> MESHVKYLDELILAIKDLNSGVDSKVQIKKVPTDPSSSQEYAKSLKILNTLIRNLKDQRRNNIMKNDTIFSKTVSALALLLEYNPFLLVMKDSNGNFEIQRLIDDFLNISVLNYDNYHRIWFMRRKLGSWCKACVEFYGKPAKFQLTAHFENTMNLYEQALTEVLLGKTELLKFYDTLKGLYILLYWFTSEYSTFGNSIAFLDSSLGFTKFDFNFQRLIRIVLYVFDSCELAALEYAEIQLKYISLVVDY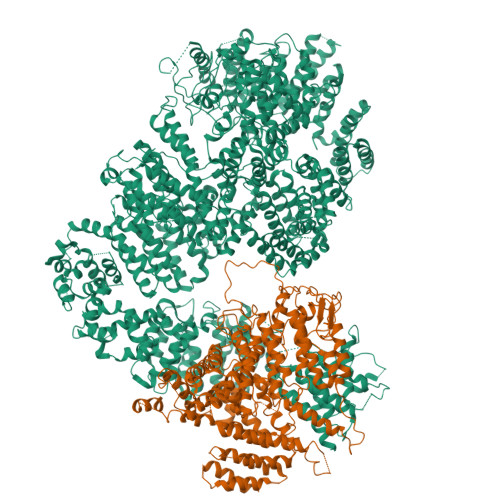VCNRTISTALDAPALVCCEQLKFVLTTMHHFLDNKYGLLDNDPTMAKGILRLYSLCISNDFSKCFVDHFPIDQWADFSQSEHFPFTQLTNKALSIVYFDLKRRSLPVEALKYDNKFNIWVYQSEPDSSLKNVTSPFDDRYKQLEKLRLLVLKKFNKTERGTLLKYRVNQLSPGFFQRAGNDFKLILNEASVSIQTCFKTNNITRLTSWTVILGRLACLESEKFSGTLPNSTKDMDNWYVCHLCDIEKTGNPFVRINPNRPEAAGKSEIFRILHSNFLSHPNIDEFSESLLSGILFSLHRIFSHFQPPKLTDGNGQINKSFKLVQKCFMNSNRYLRLLSTRIIPLFNISDSHNSEDEHTATLIKFLQSQKLPVVKENLVIAWTQLTLTTSNDVFDTLLLKLIDIFNSDDYSLRIMMTLQIKNMAKILKKTPYQLLSPILPVLLRQLGKNLVERKVGFQNLIELLGYSSKTILDIFQRYIIPYAIIQYKSDVLSEIAKIMCDGDTSLINQMKVNLLKKNSRQIFAVALVKHGLFSLDILETLFLNRAPTFDKGYITAYLPDYKTLAEITKLYKNSVTKDASDSENANMILCSLRFLITNFEKDKRHGSKYKNINNWTDDQEQAFQKKLQDNILGIFQVFSSDIHDVEGRTTYYEKLRVINGISFLIIYAPKKSIISALAQISICLQTGLGLKEVRYEAFRCWHLLVRHLNDEELSTVIDSLIAFILQKWSEFNGKLRNIVYSILDTLIKEKSDLILKLKPYTTLALVGKPELGILARDGQFARMVNKIRSTTDLIPIFANNLKSSNKYVINQNLDDIEVYLRRKQTERSIDFTPKKVGQTSDITLVLGALLDTSHKFRNLDKDLCEKCAKCISMIGVLDVTKHEFKRTTYSENEVYDLNDSVQTIKFLIWVINDILVPAFWQSENPSKQLFVALVIQESLKYCGLSSESWDMNHKELYPNEAKLWEKFNSVSKTTIYPLLSSLYLAQSWKEYVPLKYPSNNFKEGYKIWVKRFTLDLLKTGTTENHPLHVFSSLIREDDGSLSNFLLPYISLDIIIKAEKGTPYADILNGIIIEFDSIFTCNLEGMNNLQVDSLRMCYESIFRVFEYCKKWATEFKQNYSKLHGTFIIKDTKTTNMLLRIDEFLRTTPSDLLAQRSLETDSFERSALYLEQCYRQNPHDKNQNGQLLKNLQITYEEIGDIDSLDGVLRTFATGNLVSKIEELQYSENWKLAQDCFNVLGKFSDDPKTTTRMLKSMYDHQLYSQIISNSSFHSSDGKISLSPDVKEWYSIGLEAANLEGNVQTLKNWVEQIESLRNIDDREVLLQYNIAKALIAISNEDPLRTQKYIHNSFRLIGTNFITSSKETTLLKKQNLLMKLHSLYDLSFLSSAKDKFEYKSNTTILDYRMERIGADFVPNHYILSMRKSFDQLKMNEQADADLGKTFFTLAQLARNNARLDIASESLMHCLERRLPQAELEFAEILWKQGENDRALKIVQEIHEKYQENSSVNARDRAAVLLKFTEWLDLSNNSASEQIIKQYQDIFQIDSKWDKPYYSIGLYYSRLLERKKAEGYITNGRFEYRAISYFLLAFEKNTAKVRENLPKVITFWLDIAAASISEAPGNRKEMLSKATEDICSHVEEALQHCPTYIWYFVLTQLLSRLLHSHQSSAQIIMHILLSLAVEYPSHILWYITALVNSNSSKRVLRGKHILEKYRQHSQNPHDLVSSALDLTKALTRVCLQDVKSITSRSGKSLEKDFKFDMNVAPSAMVVPVRKNLDIISPLESNSMRGYQPFRPVVSIIRFGSSYKVFSSLKKPKQLNIIGSDGNIYGIMCKKEDVRQDNQYMQFATTMDFLLSKDIASRKRSLGINIYSVLSLREDCGILEMVPNVVTLRSILSTKYESLKIKYSLKSLHDRWQHTAVDGKLEFYMEQVDKFPPILYQWFLENFPDPINWFNARNTYARSYAVMAMVGHILGLGDRHCENILLDIQTGKVLHVDFDCLFEKGKRLPVPEIVPFRLTPNLLDALGIIGTEGTFKKSSEVTLALMRKNEVALMNVIETIMYDRNMDHSIQKALKVLRNKIRGIDPQDGLVLSVAGQTETLIQEATSEDNLSKMYIGWLPFW;> MRRETVGEFSSDDDDDILLELGTRPPRFTQIPPSSAALQTQIPTTLEVTTTTLNNKQSKNDNQLVNQLNKAQGEASMLRDKINFLNIEREKEKNIQAVKVNELQVKHLQELAKLKQELQKLEDEKKFLQMEARGKSKREVITNVKPPSTTLSTNTNTITPDSSSVAIEAKPQSPQSKKRKISDNLLKKNMVPLNPNRIIPDETSLFLESILLHQIIGADLSTIEILNRLKLDYITEFKFKNFVIAKGAPIGKSIVSLLLRCKKTLTLDRFIDTLLEDIAVLIKEISVHPNESKLAVPFLVALMYQIVQFRPSATHNLALKDCFLFICDLIRIYHHVLKVPIHESNMNLHVEPQIFQYELIDYLIISYSFDLLEGILRVLQSHPKQTYMEFFDENILKSFEFVYKLALTISYKPMVNVIFSAVEVVNIITSIILNMDNSSDLKSLISGSWWRDCITRLYALLEKEIKSGDVYNENVDTTTLHMSKYHDFFGLIRNIGDNELGGLISKLIYTDRLQSVPRVISKEDIGMDSDKFTAPIIGYKMEKWLLKLKDEVLNIFENLLMIYGDDATIVNGEMLIHSSKFLSREQALMIERYVGQDSPNLDLRCHLIEHTLTIIYRLWKDHFKQLREEQIKQVESQLIMSLWRFLVCQTETVTANEREMRDHRHLVDSLHDLTIKDQASYYEDAFEDLPEYIEEELKMQLNKRTGRIMQVKYDEKFQEMARTILESKSFDLTTLEEADSLYISMGL> GEGQQHHLGGAKQA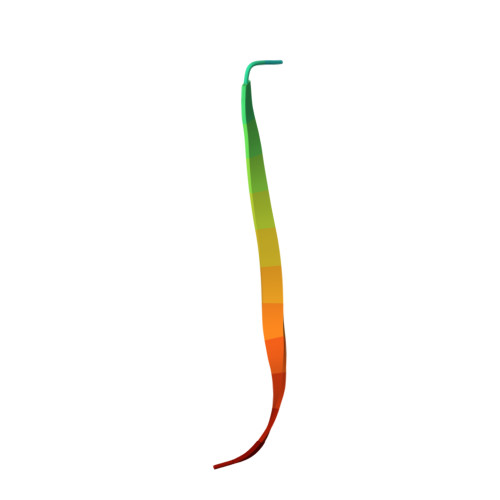GDV>[2x]HHHHHHSSGLVPRGSHMAISHVQLFSVPVSDQEKAKDFY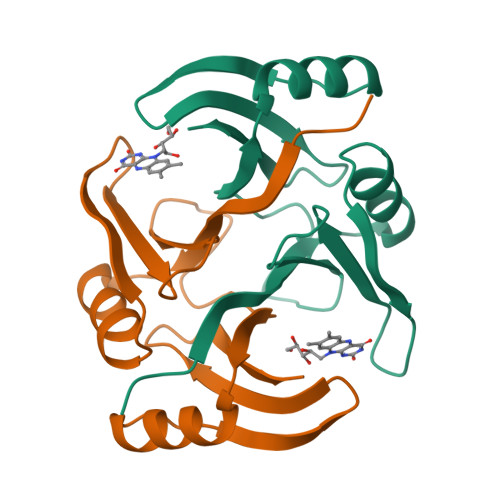VETVGFDLLADQPGVHGRWLQVAPKGADTSLVLVDWFPTMPPGSLRGLLLRTDDVDADCARLQERGVAVDGPKNTPWGRQAMFSDPDGNVIGLNQPSASAG> MDAKARNCLLQHREALEKDIKTSYIMDHMISDGFLTISEEEKVRNEPTQQQRAAMLIKMILKKDNDSYVSFYNALLHEGYKD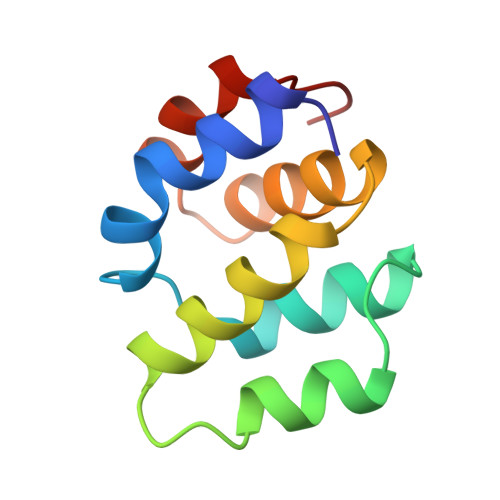LAALLHDGIPVVS> MDSASKEETLEKLDQEITVNLQKIDSNLSFCFHKITQDIIPHVATYSEICERIMDSTEWLGTMFQETGLVNLQANAAAPVGNAPVKSLVSNNVGIFPTSAEEASRQSQTDNGPNEADSAVHVNRDVHSMFNNDSIDDFHTANITSTGQILKLPDSSDEDTGSEAVPSREQTDLTGEGHGGADDEQDESTIQRQSRKRKISLLLQQQYGSSSSMVPSPIVPNKMRKQLAHEEHINNDGDNDDENSNNIESSPLKQGHHHPKGQADDNNEGPDE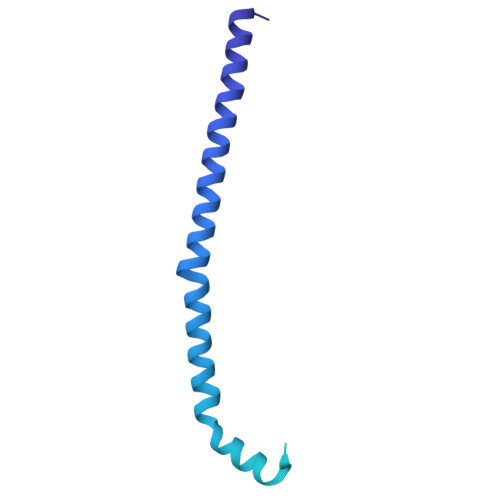EESTKEVPKPGTIIHFSTNR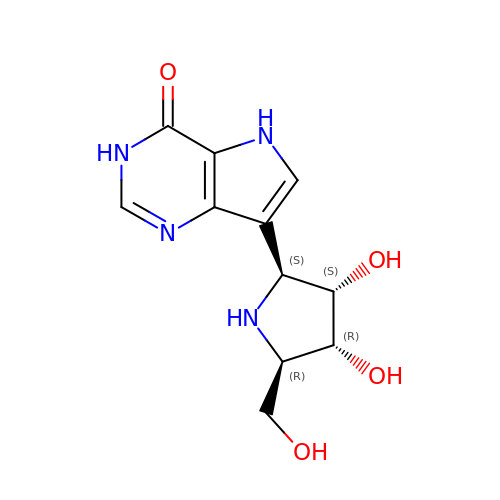1,4-DIDEOXY-4-AZA-1-(S)-(9-DEAZAHYPOXANTHIN-9-YL)-D-RIBITOL | C11 H14 N4 O4 | IWKXDMQDITUYRK-KUBHLMPHSA-N> MTAKDDYPSLSFQQDYVYIFSSDFQLSEELGVALINALSAKEIVPERLYVMLNDKTISFSFISKNKKSKNRVLSTEKKLNYKHISEYIVNEIEY;> MGSSHHHHHHSQDPVHFYETSYKYQAAD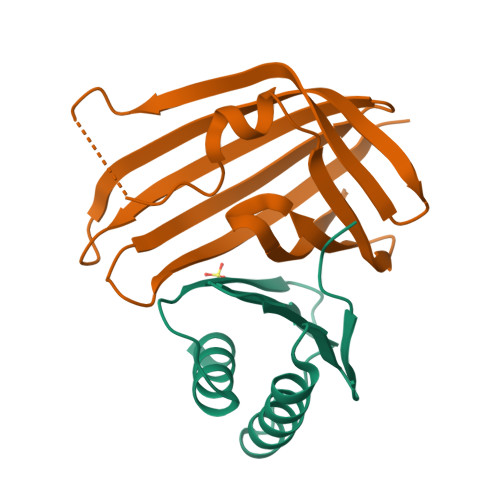STYMHDVAINVSIKGNHFTSDIIIRELVKSENKNYYNVIGHGDIIQKNTHQYYLNFDNIDVYTGTNKANMKPYKEPTSISSLINKSNNIRVVYLSEEYVVVEFFFYDGQIITLHRY>AYTTFSQTKNDQLKEPMFFGQPVNVARYDQQKYDIFEKLIEKQLSFFWRPEEVDVSRDRIDYQALPEHEKHIFISNLKYQTLLDSIQGRSPNVALLPLISIPELETWVETWAFSETIHSRSYTHIIRNIVNDPSVVFDDIVTNEQIQKRAEGISSYYDELIEMTSYWHLLGEGTHTVNGKTVTVSLRELKKKLYLCLMSVNALEAIRFYVSFACSFAFAERELMEGNAKIIRLIARDEALHLTGTQHMLNLLRSGADDPEMAEIAEECKQECYDLFVQAAQQEKDWADYLFRDGSMIGLNKDILCQYVEY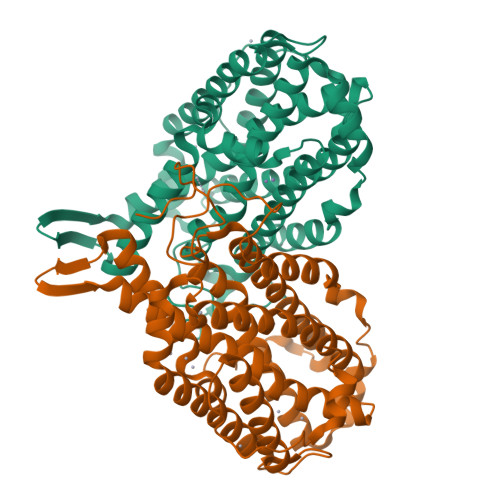ITNIRMQAVGLDLPFQTRSNPIPWINTWLVSDNVQVAPQEVEVSSYLVGQIDSEVDTDDLSNFQL[2x]> SAGINYVQNYNGNLGDFTYDESAGTFSMYWEDGVSSDFVVGLGWTTGSSNAITYSAEYSASGSSSYLAVYGWVNYPQAEYYIVEDYGDYNPCSSATSLGTVYSDGSTYQVCTDTRTNEPSITGTSTFTQYFSVRESTRTSGTVT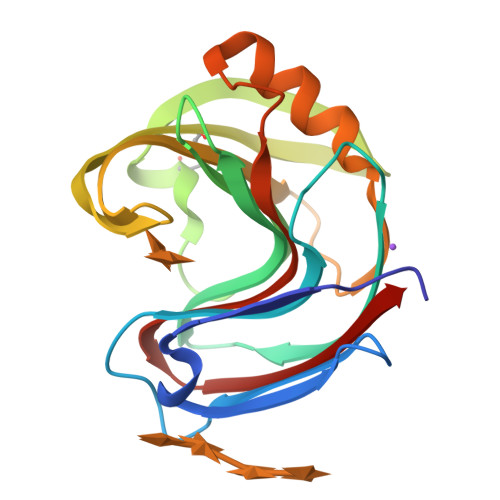VANHFNFWAQHGFGNSDFNYQVVAVAAWSGAGSASVTISS> MGDT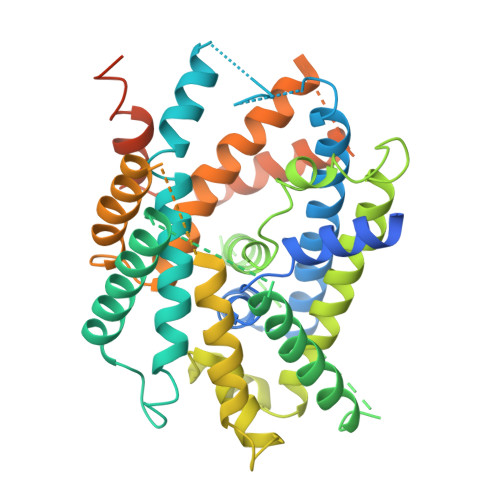GLRKRREDEKSIQSQEPKTTSLQKELGLISGISIIVGTIIGSGIFVSPKSVLSNTEAVGPCLIIWAACGVLATLGALCFAELGTMITKSGGEYPYLMEAYGPIPAYLFSWASLIVIKPTSFAIICLSFSEYVCAPFYVGCKPPQIVVKCLAAAAILFISTVNSLSVRLGSYVQNIFTAAKLVIVAIIIISGLVLLAQGNTKNFDNSFEGAQLSVGAISLAFYNGLWAYDGWNQLNYITEELRNPYRNLPLAIIIGIPLVTACYILMNVSYFTVMTATELLQSQAVAVTFGDRVLYPASWIVPLFVAFSTIGAANGTCFTAGRLIYVAGREGHMLKVLSYISVRRLTPAPAIIFYGIIATIYIIPGDINSLVNYFSFAAWLFYGLTILGLIVMRFTRKELERPIKVPVVIPVLMTLISVFLVLAPIISKPTWEYLYCVLFILSGLLFYFLFVHYKFGWAQKISKPITMHLQMLMEVVPPEEDPE> MGVVSERLYNGIVKENATFVQVLGMCPTLAVTTSAIN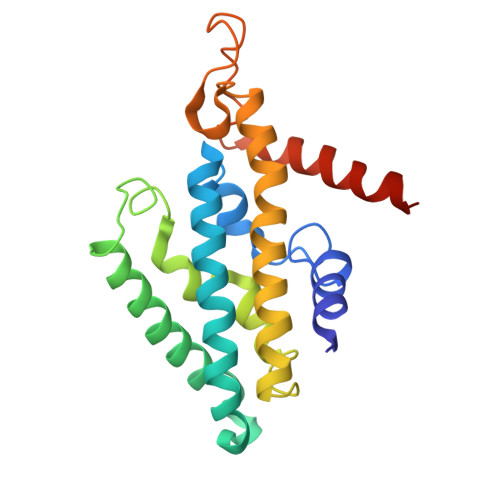GIGMGLSATVVLIGSNVVISLLKKVIPDEIRIPAYITVIATLVTVLQFLLQAYLPDLNKSLGIFIPLIVVNCIILGRAEAYANKNSVGASFFDGLGMGLGFTVSLAALGIIREFLGTGKVFGAQITPDAFQPALIMILAPGGFFTLGILMAILNQRKLKKAKAK> SKSKDRKY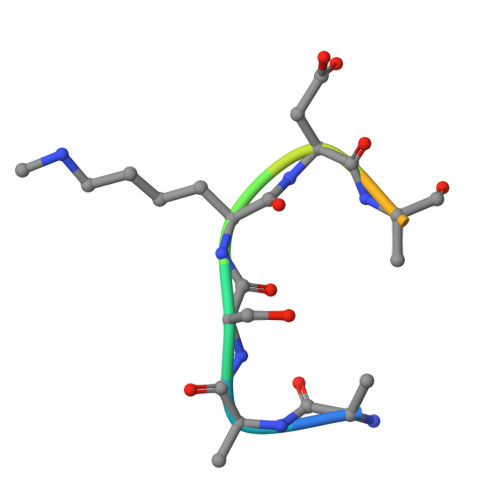TL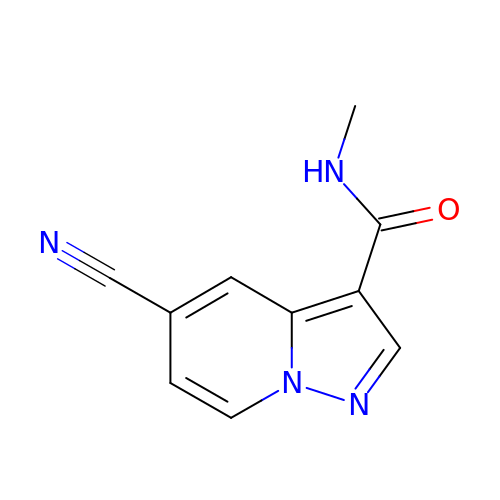5-cyano-~{N}-methyl-pyrazolo[1,5-a]pyridine-3-carboxamide | C10 H8 N4 O | RRLLSCMBISBGGI-UHFFFAOYSA-N> MILKRAYDVTPQKISTDK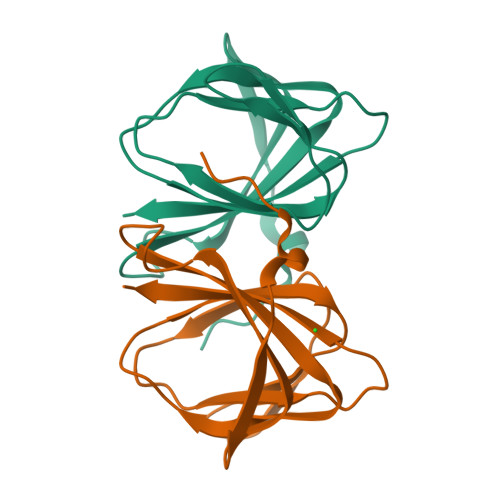VRGVRKRVLIGLKDAPNFVMRLFTVEPGGLIDRHSHPWEHEIFVLKGKLTVLKEQGEETVEEGFYIFVEPNEIHGFRNDTDSEVEFLQLIPKEGGE N-[6-[[9-(dimethylamino)-12H-benzo[a]phenoxazin-5-yl]amino]hexyl]-4-(2-oxidanyl-6-oxidanylidene-cyclohexen-1-yl)carbonyl-3-[oxidanyl(oxidanylidene)-$l^4-azanyl]benzamide 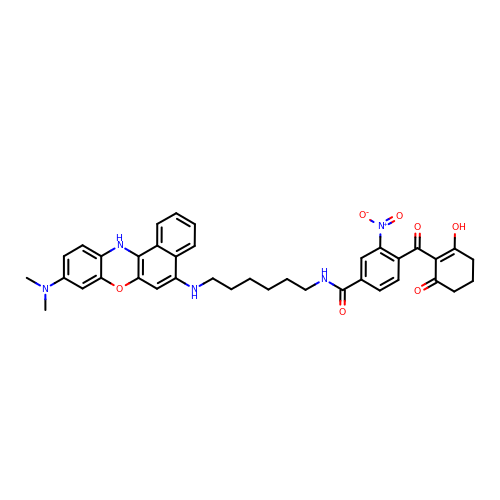| C38 H39 N5 O7 | JKNRGQRJDMEUPO-UHFFFAOYSA-N>GSHMNKLVVLGSVNADHVLQVPSFPRPGETLHGRNYQVIPGGKGANQAVAAARMQADVGFIACVGDDSFGINIRESFKLDGINTAGVKLQPNCPTGIAMIQVSDSGENSICISAEANAKLTAAAIEPDLAAIRDARYLLMQLETPLDGILKAAQEAKTAKTNVILNPAPARELPDELLKCVDLITPNETEAEVLTGITVYDDSSAQQAADALHCKGIEIVIITLGSKGVWLSQNGRGQRIPGFVVKATDTTAAGDTFNGALVTGLLQEMPLESAIKFAHAAAAISVTRFGAQTSIPTRAEVEA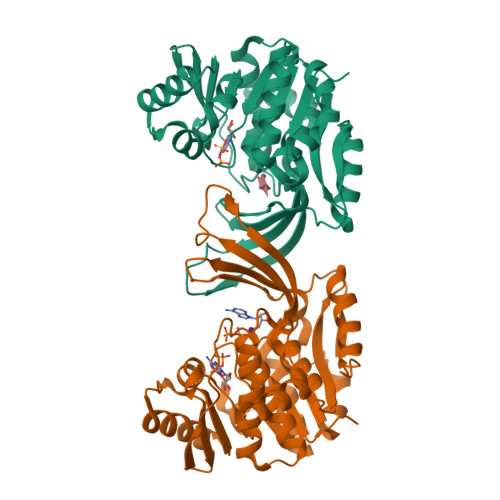FLAEHS[4x]> GAACGACAAAGA;> CGTCGACTC;> TCTACG;> TCGAGTCGTTGTCGT

In this work, we exhaustively probe the ability of all 36 immobile HJ sequences to form DNA crystals in two different designed systems. Three separate self-assembling DNA crystal systems are described in this report: the “4 × 5” and “4 × 6” designs (collectively referred to as the 4 × N systems), and a third construct with a “scrambled” sequence variant of the 4 × 6 lattices. Self-assembly was mediated by three constituent oligonucleotides: (S1) containing four sequence repeats of either 5 or 6 bases; (S2) composed of 21 bases containing complementary regions to both (S1); and (S3) which forms the second junction crossover. The HJ serves as the fundamental component at the core of each unit, and the ultimate assembly of the full lattice is facilitated by the complementary 2-base sticky ends that tail each duplex.

To investigate this possibility, we designed “scrambled” sequences with targeted base substitutions, while maintaining GC content, along each “stem”. Contrary to the buffer preference observed with the native P32 crystals, the scrambled systems exhibited an exclusive preference towards low salt buffers, much like the native R3 crystals. Remarkably, only J1 and J2 retained the P32 symmetry, with all others yielding an R3 lattice. There appeared to be only a marginal difference in the average cell lengths in the R3 scramble crystals (a = b = 113.04 c = 51.10) relative to the native 4 × 6 sequences: the a, b axis trended ~2 Å shorter and c ~1.3 Å longer, whereas in the J1 and J2 cases, the crystals were in good agreement with the original 4 × 6 motif. The average angles of the R3 and P32 crystals were 61.00° (σ = 1.21) and 58.05° (σ = 1.39), respectively. The role of longer-range sequence effects on junction angles remains a largely open question, but the effect in our crystal system is significant. However, in the majority of the crystal structures reported here, the cacodylate anion indeed fits best into the electron density map of our X-ray structures, due to the presence of sodium cacodylate in the crystallization solution.> MALTLAMVQRHLQADLIEDDERSYVMEQLLPAARESAEMFLNRNIYSTSEELAAAVAAGTAGQYPLVTPRAVEQAILLMLGDFYRDREATGKPVSTSAHNLLYPYRVKV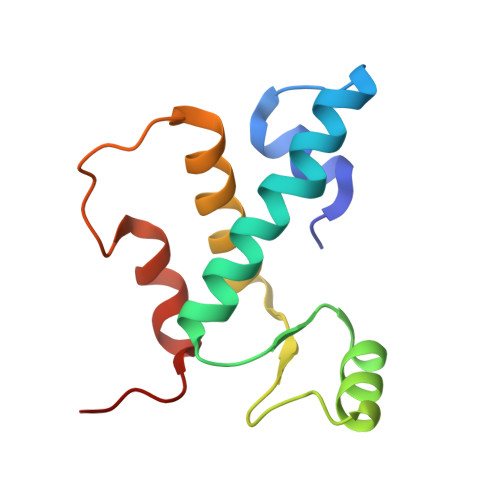GV>AIDEIKSRGYLLVGLSADFPPFEFVDENGNIVGFDVDLAKEIARRLGVELKIVDMTWDGLIPSLLTKKIDVIISGMTITEERKKVVAFSDPYFDAGGGGSGEQYGIAVRKEDTDLLEFINSVLRELKKLEHHHHHH[2x]

In the last few years, we have characterized the arginine-binding protein isolated from the hyperthermophilic organism Thermotoga maritima (TmArgBP). Although substrate-binding proteins are generally monomeric, TmArgBP is essentially dimeric, with the concomitant presence, as minor components, of higher oligomerization states. The three-dimensional structure of the protein has also shown that the arginine binding does not only produce a remarkable tertiary structure variation of TmArgBP but also a radical rearrangement of its quaternary structure. The biophysical characterization of the protein has also revealed that it is endowed with an unusual stability against temperature, chemical denaturants and pressure.

Although both domains cooperate to the anchoring of the arginine in the wild-type protein, only D1 is able to bind this ligand when considered as isolated entity. Due to the different numbering scheme adopted for TmArgBP D1 (see the notations section in the Materials and Methods), the mutation is F57W and the mutant is denoted thereafter D1F57W. The domain was successfully crystallized and diffraction data were collected at 1.79 Å resolution. The asymmetric unit of the crystals contains two copies of the domain whose structure is very similar both at local and at global level (the RMSD value of the two copies is 0.31 Å). A comparative analysis of the global structure of D1F57W with previous structural characterizations of D1 in different binding states or embodied in the native protein indicates that the mutation does not produce major rearrangements. The inspection of the binding pocket indicates that the arginine is anchored by a remarkable number of residues that establish a variety of different interactions with the ligand. A remarkable contribution to the recognition of arg is provided by the mutated residue W57. The values of the side chain dihedral angles (χ1; χ2) that the residue adopts in the crystallographic structure are (−178.16°, −92.18°) and (174.49°, −108.34°) for the two molecules present in the asymmetric unit. This observation indicates that W57 assumes the rotameric state predicted by the computational analysis reported above. Notably, the accessible surface area of this residue decreases from 104.9 Å2, in the absence of the ligand, to 31.6 Å2. The drastic change in the local environment of the tryptophan explains the variation of the fluorescence signal associated with the arginine binding.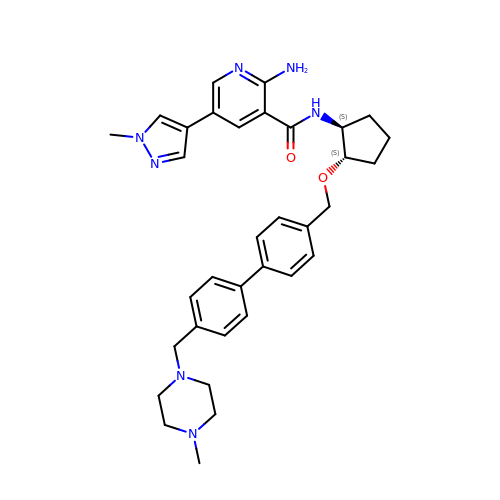2-azanyl-~{N}-[(1~{S},2~{S})-2-[[4-[4-[(4-methylpiperazin-1-yl)methyl]phenyl]phenyl]methoxy]cyclopentyl]-5-(1-methylpyrazol-4-yl)pyridine-3-carboxamide | C34 H41 N7 O2 | GTVWQFJFCAUNFY-ACHIHNKUSA-N6-(2,6-dichlorophenyl)-2-({4-[2-(diethylamino)ethoxy]phenyl}amino)-8-methylpyrido[2,3-d]pyrimidin-7(8H)-one 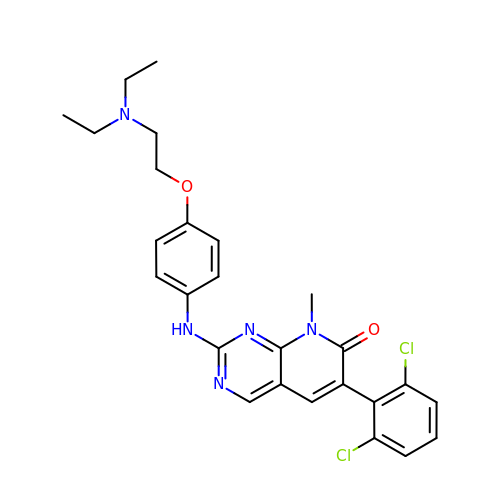| C26 H27 Cl2 N5 O2 | IFPPYSWJNWHOLQ-UHFFFAOYSA-N>[2x]AFELPSLPYAIDALEPHISKETLEFHHGKHHNTYVVKLNGLIPGTKFENKSLE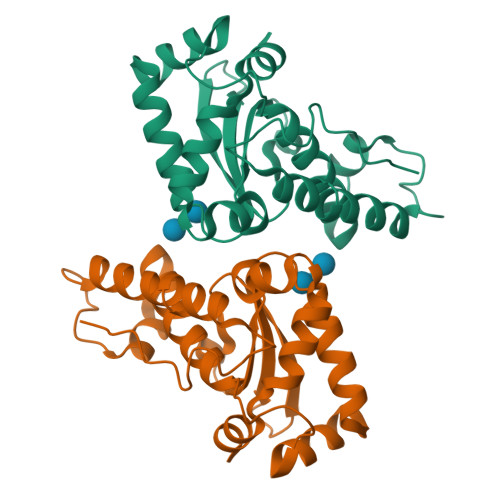EIVCSSDGGVFNNAAQIWNHTFYWNSLSPNGGGAPTGAVADAINAKWGSFDAFKEALNDKAVNNFGSSWTWLVKLADGSLDIVNTSNAATPLTDDGVTPILTVDLWEHAYYIDYRNVRPDYLKGFWSLVNWEFANANFA> 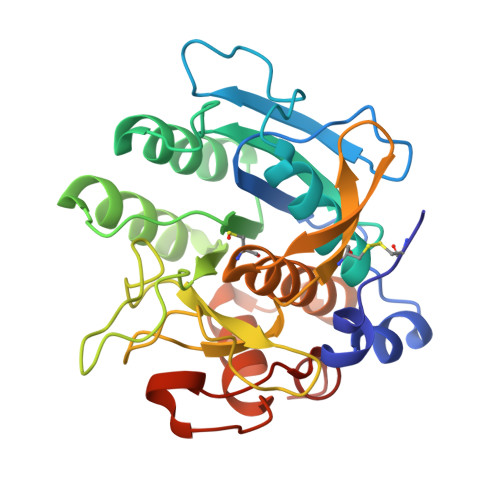AKCVSYGVSQIKAPALHSQGYTGSNVKVAVIDSGIDSSHPDLNVAGGASFVPSETNPFQDNNSHGTHVAGTVLAVAPSASLYAVKVLGADGSGQYSWIINGIEWAIANNMDVINMSLGGPSGSAALKAAVDKAVASGVVVVAAAGNSGTSGSSSTVSYPAKYPSVIAVGAVDSSNQRAPWSSVGPELDVMAPGVSICSTLPGNKYGAHSGTCPASNHVAGAAALILSKHPNWTNTQVRSSLENTATKLGDSFYYGKGLINVEAAAQHHHHHH>SRCTHLENRDFVTGTQGTTRVTLVLELGGCVTITAEGKPSMDVWLDAIYQENPAKTREYCLHAKLSDTKVAARCPTMGPATLAEEHQGGTVCKRDQSDRGHGNHCGLFGKGSIVACVKAACEAKKKATGHVYDANKIVYTVKVEPHTGDYVAANETHSGRKTASFTISSEKTILTMGEYGDVSLLCRVASGVDLAQTVILELDKTVEHLPTAWQVHRDWFNDLALPWKHEGAQNWNNAERLVEFGAPHAVKMDVYNLGDQTGVLLKALAGVPVAHIEGTKYHLKSGHVTCEVGLEKLKMKGLTYTMCDK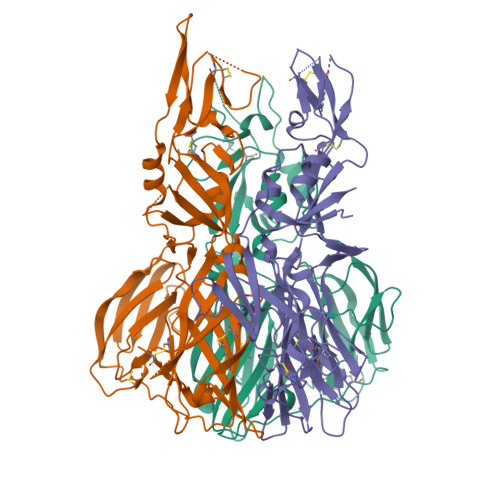TKFTWKRAPTDSGHDTVVMEVTFSGTKPCRIPVRAVAHGSPDVNVAMLITPNPTIENNGGGFIEMQLPPGDNIIYVGELSHQWFQKGSSIGRVFQGGGSGGGSGGFLSSIGKAVHTVLGGAFNSIGPFEDDDDKAGWSHPQFEK[3x]> AAHGSNPEQLKHCNGILKELLSKKHAAYAWPFYKPVD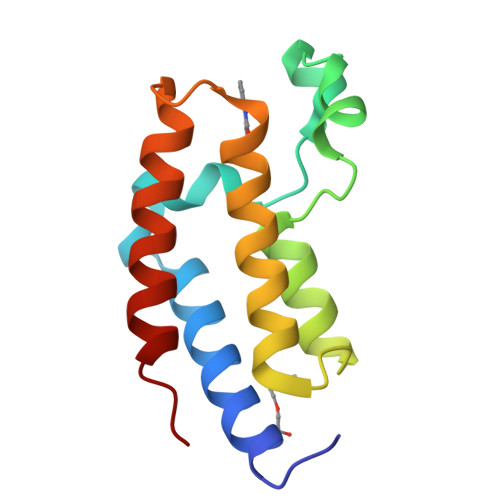ASALGLHDYHDIIKHPMDLSTVKRKMENRDYRDAQEFAADVRLMFSNCYKYNPPDHDVVAMARKLQDVFEFRYAKMPD(2R)-3-hydroxy-2-[(4-methoxyphenyl)sulfonylamino]-N-oxo-propanamide | C10 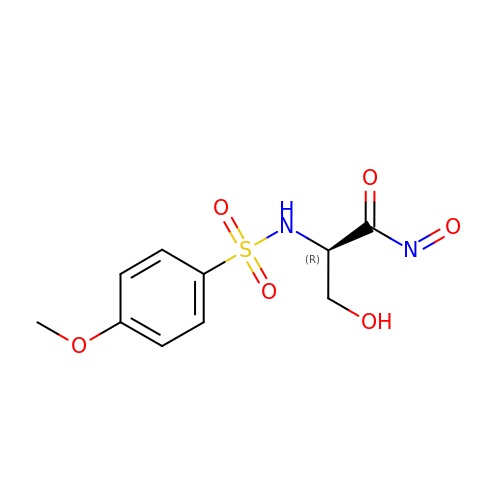H12 N2 O6 S | LPGVJAGNVVNWCU-SECBINFHSA-N{3-[(3aR,4S,5S,6aR)-5-azaniumyl-5-carboxyoctahydrocyclopenta[c]pyrrol-2-ium-4-yl]propyl}(trihydroxy)borate(1-) | C11 H24 B N2 O5 | 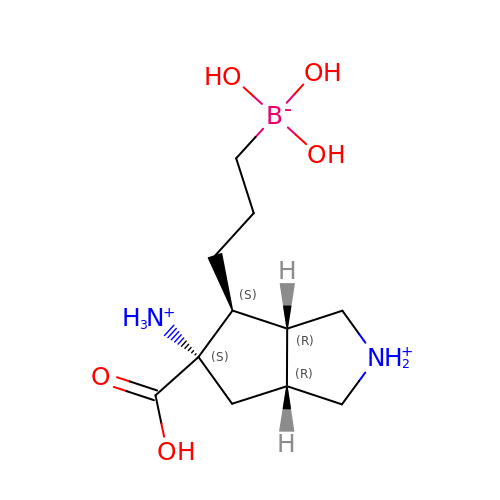WOVPMRKEMBIWOY-DKIAZLNASA-P>[12x]MVIATDDLEVACPKCE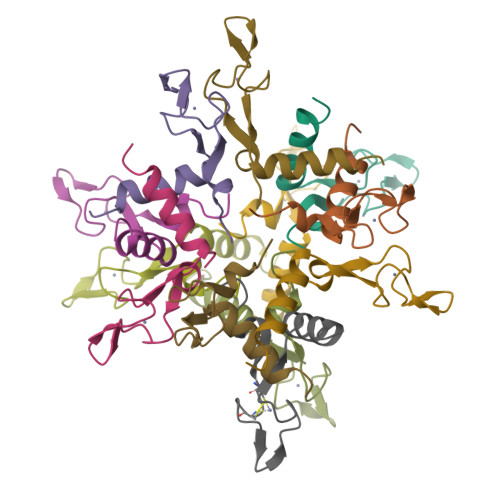RAGEIEGTPCPACSGKGVILTAQGYTLLDFIQKHLNK The Type-IV restriction endonuclease (REase)ScoA3McrA (abbreviated as ScoMcrA hereafter) catalyzes multiple double strand cleavages 16–28 nucleotides (nt) away from the phosphorothioate linkage with the core sequence GPSGCC/GPSGCC. The DNA PT-dependent REase ScoMcrA distinguishes PT-DNA from normal DNA which differs only by one oxygen-to-sulfur swap, and presumably encodes a domain to specifically recognize sulfur on PT-DNA. Each ScoMcrA protomer consists of a head domain, an uncharacterized domain, a SRA-like domain, and an HNH domain. The uncharacterized domain binds specifically to PT-DNA whose sulfur atom is in the Rp but not in the Sp configuration, therefore we named it sulfur-binding domain (SBD).

In each asymmetric unit, there are six ScoMcrA molecules, which are assembled into three dimers. Superimposition of the six ScoMcrA protomers in the asymmetric unit shows that the head domain exhibits substantial positional variance with respect to the other domains, suggesting that it is rather flexibly attached to the rest of the molecule. In the HNH domain, two β-strands and an α-helix harbor the active site residues H508, N522, and H531, that are critical for its endonuclease activity. Four cysteine residues, C484, C489, C527, and C530, coordinate a Zn2+ ion in a zinc finger-like structure. A domain sandwiched between the SBD and the HNH domain in ScoMcrA structure has an overall structure similar to classical SRA, but does not possess the NKR finger and thumb features. A comparison of ScoMcrA-SBD structures in the free and PT-DNA bound states revealed that PT-DNA binding induces a rotation of the side-chain of Y164 in the sulfur-binding cavity of ScoMcrA-SBD. When not in complex with PT-DNA, Y164 is flexible and samples a variety of conformations. Of the six ScoMcrA molecules in the asymmetric unit, only two have clearly observable electron densities for the side-chain of Y164 and both of which are in the closed states. In these two molecules, the hydrophobic phenyl ring of the side-chain of Y164 covers the opening of the non-polar sulfur-binding cavity.

>GSAPSEITRAGILQAIAEHDRIGPEAFRATYGFHAATSYFLEHEGRLYDSKAIAGVAHMYDFGVALKPSSPGLSGGLKHAVAWLRREGFTIREAPKTFHRRVGDVRPARRAMGPALHRPVLLLWAIGQAVARAPRLQPWSTTRDAVAPLMEKYGQVEDGVDGVRYPFWALVRDDLWCVEQAEELTLTSRGRRPTLESLNAVDPSAGLREDDYNLLRSQPEAAASAAAGLIARYFHLLPAGLLEDFGLHELLAGRWPDALRPLLGETFKDRDAIWRAYGGQKMAGIGCLADGILSAFSDDKGPYADGRIPDTTWIAYVGDGLSGDQKLTDGNELMAEHQAVGRALRYWHKPFQGQWSFETWAVIVQRRLRWGLGEDKLPRREFLWVLAPVPSPERETWPPEVLEALEADTGELHDDTGDYRPSDLALTPGAPDGTESDDEAYRRLAQKAEANAERRGQLKKPTVADKYVRDPSARGAVLKRCQKRCENPECAGHPTELTKAGLPILQVDHVNDLAKGGPDVPWNMIALCPNCHALKTYGANKVRLQRLLAATARRLHEEKLQ[6x]> RADQLADESLES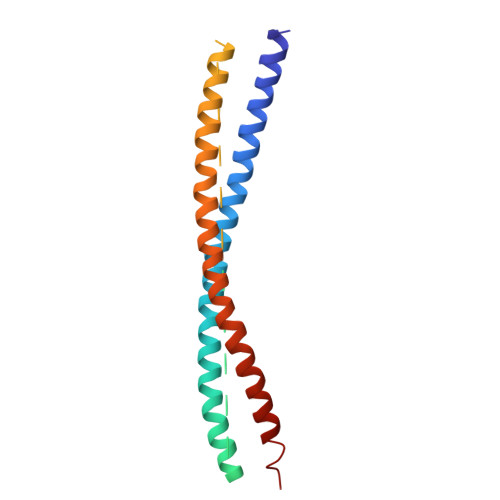TRRMLQLVEESKDAGIRTLVMLDEQGEQLDRVEEGMNHINQDMKEAEKNLKDLGKFCGLCVCPCNKLKSSDAYKKAWGNNQDGVVASQPARVVDEREQMAISGGFIRRVTNDARENEMDENLEQVSGIIGNLRHMALDMGNEIDTQNRQIDRIMEKADSNKTRIDEANQRATKMLG>[2x]MAIENRASRMREKLQKELEPVELVIEDVSYQHAGHAGMKGR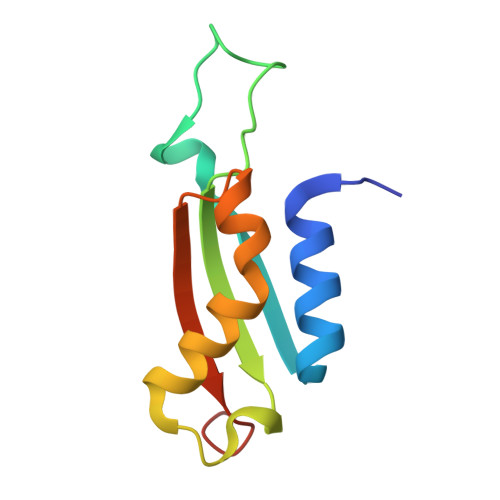TDDETHFNVKIVSKGFEGMNLVKRHRLVYHLLREELDTGLHALSIVSKTPSESPSKD>[7x]MGSSHHHHHHSQDPMKHRYSRNRLYLNPKEQELIKDYPILLGGAGIGSIIAECALRFGFENITIVDGDHVENSNLNRQNYTEGDVSVNKVEAIKARLKSINSKANIKIHNCFLT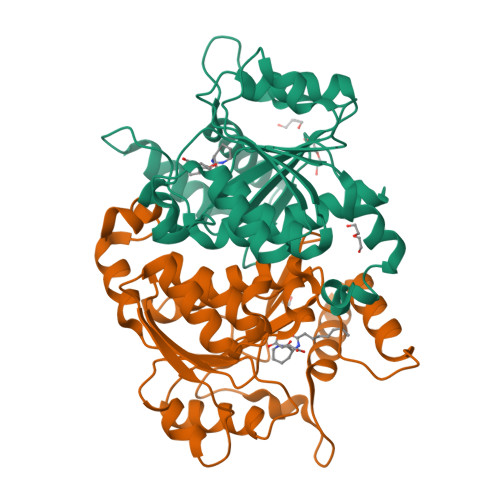SDNVEEYIKGHKVAINALDFSSEVPLLFDEICQKMDIPVLHPYNLGWGGLVTIISPKGLSLNSIAKKGEKFNELNVVEYVSSYMRFWGKPQEWLEDIIYKFKNEREKLSPPQLSVGSWVVAGMCTHILFNIATQREIKSFPEFYLSSLEG> G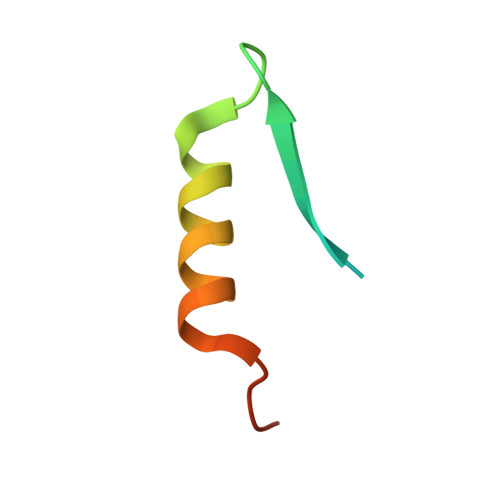EFSGLTPRSALLYKFNGSPSKSLKDINNMIRQGEQRTKKR>ADTIVAVELDTYPNTDIGDPSYPHIGIDIKSVRSKKTAKWNMQNGKVGTAHIIYNSVGKRLSAVVSYPNGDSATVSYDVDLDNVLPEWVRVGLSASTGLYKETNTILSWSFTSKLKSNSTHETNALHFMFNQFSKDQKDLILQGDATTGTEGNLRLTRVSSNGSPQGSSVGRALFYAPVHIWESSAVVASFEAT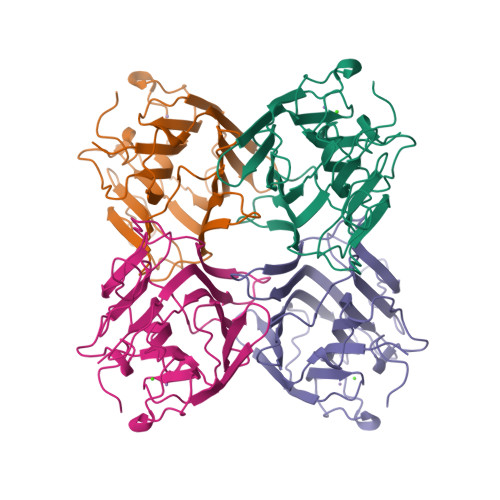FTFLIKSPDSHPADGIAFFISNIDSSIPSGSTGRLLGLFPDAN[4x]> GPLGSKNAP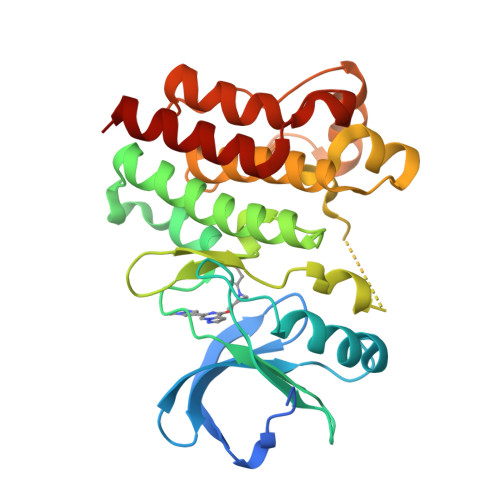STAGLGYGSWEIDPKDLTFLKELGTGQFGVVKYGKWRGQYDVAIKMIKEGSMSEDEFIEEAKVMMNLSHEKLVQLYGVCTKQRPIFIITEYMANGCLLNYLREMRHRFQTQQLLEMCKDVCEAMEYLESKQFLHRDLAARNCLVNDQGVVKVSDFGLSRYVLDDEYTSSVGSKFPVRWSPPEVLMYSKFSSKSDIWAFGVLMWEIYSLGKMPYERFTNSETAEHIAQGLRLYRPHLASEKVYTIMYSCWHEKADERPTFKILLSNILDVMDEES>[2x]M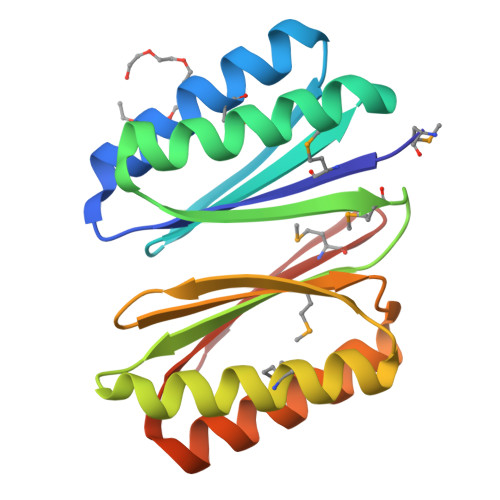GVMVIVFEGDDLEALEKALKEMIRQARKFAGTVTYTLSGNRLVIVITGVPEQVRKELAKEAERLKAEFNINVQYQIMGSGSGVMVIVFEGDDLEALEKALKEMIRQARKFAGTVTYTLSGNRLVIVITGVPEQVRKELAKEAERLKAEFNINVQYQIMTGSLEHHHHHH> MSHHHHHHHHHHDSNGIPTENLYFQGAGVAFGSFDDSFSLASLRAYLAEFISTLLFVFAGVGSAIAYAKLTSDAALDTPGLVAIAVCHGFALFVAVAIGANISGGHVNPAVTFGLAVGGQITVITGVFYWIAQLLGSTAACFLLKYVTGGLAVPTHSVAAGLGSIEGVVMEIIITFALVYTVYATAADPKKGSLGTIAPLAIGLIVGANILAAGPFSGGSMNPARSFGPAVAAGDFSGHWVYWVGPLIGGGLAGLIYGNVFMGSSEHVPLASADF

Aquaporins are integral membrane proteins that form channels that accelerate the passive permeation of small polar uncharged molecules, like water and ammonia, across lipid membranes of the cell. Tonoplast Intrinsic Proteins (TIPs) belonging to the Major Intrinsic Protein family, also known as the aquaporin (AQP) superfamily, have been shown to conduct both water and ammonia. Crystal structures have established that AQPs are homotetramers, where each of the monomers holds a functional pore created by six membrane-spanning helices (helix 1‒helix 6), five connecting loops (loop A‒loop E), and two shorter helices (helix B and helix E), both displaying the AQP-signature motif Asn-Pro-Ala (NPA). Substrate specificity is thought to be achieved by the aromatic/arginine selectivity filter, which has been defined as four residues located at the noncytosolic end of the pore.

AtTIP2;1, solubilized by n-octyl-β-D-glucoside, was crystallized at pH 5.0 and the structure determined at 1.18 Å resolution. In the reported structure, 238 amino acid residues are resolved, and only the N-terminal tag and 12 native residues at the C-terminus are not included in the model. Accordingly, the structure of AtTIP2;1 constitutes an open channel where the cytosolic and vacuolar vestibules are connected by a pore lining eight water molecules in a single file. Interestingly, the pore diameter of AtTIP2;1 at the NPA region is smaller than in other AQPs, and it remains constant at around 3 Å throughout the pore. In line with this, TIP2s deviate from other AQPs, and as expected from mutational studies and modeling, the wider selectivity filter is mainly due to an isoleucine (Ile 185) at position H5P in helix 5, replacing a histidine that is conserved in the water-specific AQPs. However, the most striking feature of the AtTIP2;1 selectivity filter arises from an unpredicted positioning of the arginine at HEP in helix E (Arg 200), a conserved residue in nearly all AQPs. In AtTIP2;1, the arginine side chain is pushed to the side of the pore by a histidine located in loop C (His 131), which now appears as a fifth residue (LCP) of an extended selectivity filter. The novel position of the arginine is further stabilized by a hydrogen bond to the histidine (His 63) at position H2P in helix 2, which occupies essentially the same space as corresponding aromatic residues of water and glycerol channels (e.g., Phe 81 in SoPIP2;1, Trp 48 in EcGlpF) without direct effects on the pore aperture. In contrast to His 63, the additional His 131 at position LCP in loop C points to the center of the pore and forms a hydrogen bond to a pore-water (Wat 2). In fact, structure and MD simulations concur that loop C leaves enough space for a continuous side pore reaching from the selectivity filter all the way to the vacuolar surface.>AVVPPAGTPWGTAYDKAKAALAKLNLQDKVGIVSGVGWNGGPCVGNTSPASKISYPSLCLQDGPLGVRYSTGSTAFTPGVQAASTWDVNLIRERGQFIGEEVKASGIHVILGPVAGPLGKTPQGGRNWEGFGVDPYLTGIAMGQTINGIQSVGVQATAKHYILNEQELNRETISSNPDDRTLHELYTWPFADAVQANVASVMCSYNKVNTTWACEDQYTLQTVLKDQLGFPGYVMTDWNAQHTTVQSANSGLDMSMPGTDFNGNNRLWGPALTNAVNSNQVPTSRVDDMVTRILAAWYLTGQDQAGYPSFNISRNVQGNHKTNVRAIARDGIVLLKNDANILPLKKPASIAVVGSAAIIGNHARNSPSCNDKGCDDGALGMGWGSGAVNYPYFVAPYDAINTRASSQGTQVTLSNTDNTSSGASAARGKDVAIVFITADSGEGYITVEGNAGDRNNLDPWHNGNALVQAVAGANSNVIVVVHSVGAIILEQILALPQVKAVVWAGLPSQESGNALVDVLWGDVSPSGKLVYTIAKSPNDYNTRIVSGGSDS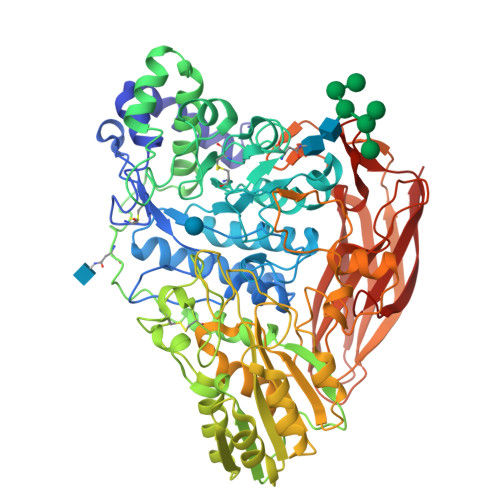FSEGLFIDYKHFDDANITPRYEFGYGLSYTKFNYSRLSVLSTAKSGPATGAVVPGGPSDLFQNVATVTVDIANSGQVTGAEVAQLYITYPSSAPRTPPKQLRGFAKLNLTPGQSGTATFNIRRRDLSYWDTASQKWVVPSGSFGISVGASSRDIRLTSTLSVA[2x]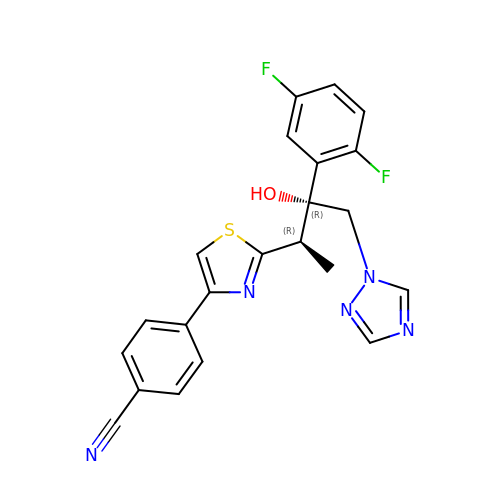4-{2-[(2R,3R)-3-(2,5-difluorophenyl)-3-hydroxy-4-(1H-1,2,4-triazol-1-yl)butan-2-yl]-1,3-thiazol-4-yl}benzonitrile | C22 H17 F2 N5 O S | DDFOUSQFMYRUQK-RCDICMHDSA-N> MTLIENLNSDKTFLENNQYTDEGVKVYEFIFGENYISSGGLEATKKILSDIELNENSKVLDIGSGLGGGCMYINEKYGAHTHGIDICSNIVNMANERVSGNNKIIFEANDILTKEFPENNFDLIYSRDAILALSLENKNKLFQKCYKWLKPTGTLLITDYCATEKENWDDEFKEYV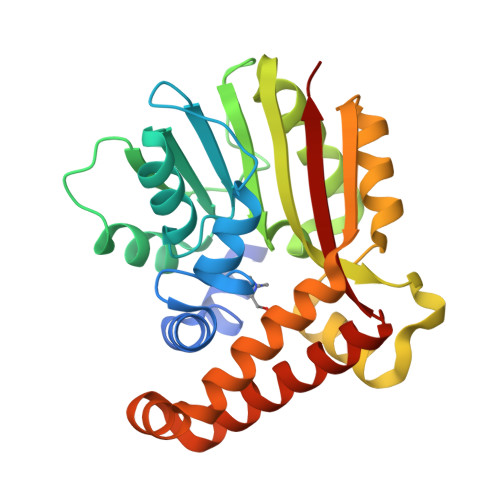KQRKYTLITVEEYADILTACNFKNVVSKDLSDYWNQLLEVEHKYLHENKEEFLKLFSEKKFISLDDGWSRKIKDSKRKMQRWGYFKATKN>[3x]MQSDTQEANDIVTLANLQYNGSTPADAFETKVTNIIDRLNNNGIHINNKVACQLIMRGLSGEYKFLRYTRHRHLNMTVAELFLDIHAIYEEQQGSRNPLEHHHHHH

Excessive replication of Saccharomyces cerevisiae Ty1 retrotransposons is regulated by Copy Number Control, a process requiring the p22/p18 protein produced from a sub-genomic transcript initiated within Ty1 GAG. To minimize genomic damage, p22/p18 interrupts virus-like particle function by interaction with Gag. Thus, p22 is identical to the C-terminal half of Gag-p49 and is processed at the C-terminus by PR to generate a mature protein p18, that is identical to the C-terminal half of mature capsid Gag-p4525,27. The structure comprises an all α-helical domain related to that observed in the CA-CTD of the yeast Ty3 retrotransposon, ARC proteins, and orthoretroviruses.

We determined the crystal structures of p18mAUG1 and p18mAUG2 expressed in E. coli. The p18mAUG2 structure was solved by multi-wavelength anomalous diffraction (MAD) using crystals of Se-Met substituted protein. In both structures, the asymmetric unit (ASU) comprises three copies of the p18m monomer. The structural superposition of all six copies, three from the p18mAUG1 structure and three from the p18mAUG2 structure, have an RMSD of <0.25 Å for all pairwise alignments overall Cα atom positions. There is no additional density for residues 249 to 259 that constitute the additional N-terminal sequence difference between AUG1 and AUG2. Therefore, we consider both structures to be identical, and define p18m as residues M259-N355 (p18mAUG2) and representing the minimal domain required for CNC activity. The co-expression results show that regions of Gag required for CNC comprise residues M249-N355 in p18mAUG1 or M259-N355 in p18mAUG2 and imply that the nucleic acid chaperone domain of Gag is not required for CNC. Inspection of the p18m crystal structures revealed three monomers in the ASU, each forming two dimer interfaces. Dimer-1 involves a largely hydrophobic interaction between the exposed surfaces of α1 and α3 on two opposing monomers whereas the Dimer-2 interaction is through the side chains of residues exposed on the exterior of α4 and α5. The application of this model gave a much-improved best fit that comprised p18m monomers in a tightly associating monomer-dimer equilibrium, KD(1-2) of 0.73 µM, together with a weakly associating dimer-tetramer equilibrium, KD(2-4) of 43.2 µM.> MGHMPERFDAFICYCPSDIQFVQEMIRQLEQTNYRLKLCVSDRDVLPGTCVWSIASELIEKRCRRMVVVVSDDYLQSKECDFQTKFALSLSPGAHQKRLIPIKYKAMKKEFPSILRFITVCDYTNPCTKSWFWTRLAKALSLPLEHHHHHH

MyD88 and MAL are Toll-like receptor (TLR) adaptors that signal to induce pro-inflammatory cytokine production. We previously observed that the TIR domain of MAL (MALTIR) forms filaments in vitro and induces formation of crystalline higher-order assemblies of the MyD88 TIR domain (MyD88TIR). Here, we present MicroED and SFX structures of the MyD88TIR assembly, which reveal a two-stranded higher-order assembly arrangement of TIR domains analogous to that seen previously for MALTIR. We demonstrate via mutagenesis that the MyD88TIR assembly interfaces are critical for TLR4 signaling in vivo, and we show that MAL promotes unidirectional assembly of MyD88TIR.

The MyD88TIR microcrystals were studied in parallel using SFX. By using a micro-focused beam (nominally 1 × 1 µm full width at half maximum (FWHM)), and optimizing crystal concentration (7.5 × 108 crystals/ml), high-quality diffraction patterns from individual crystals were collected. Overall, the SFX dataset comprised 4725 indexed patterns from 13,528 hits (35% indexing rate) out of 1,029,868 detector frames (average hit rate of 1.3%). To enable a direct comparison between the MicroED and SFX models, we also solved, rebuilt and refined the SFX MyD88TIR structure using an identical protocol as described for the MicroED data (SFXb). The MicroED and SFXb MyD88TIR structures, which were built and refined using the same protocol, are almost identical, with a root mean square deviation (RMSD) of 0.4 Å for 138 Cα atoms. Minor differences in some side-chain conformations can be observed, which is most likely due to the flexibility of certain regions resulting in poorly defined electron density or as a result of the difference in the data collection temperature. The lattice parameters derived from the SFX data were found to be slightly larger than in the MicroED data collected under cryo-conditions. Our room-temperature SFX data also showed a slight increase in lattice parameters along the a-axis, when compared to the cryogenic MicroED data, indicating the lattice change is related to the temperature difference between the two data sets. In our investigation, only subtle differences were observed between the MicroED and SFX structures, which may be explained by the differences in the data resolution and completeness, flexibility of certain regions, and difference between cryogenic and room temperature data collection.> MSGIALSRLAQERKAWRKDHPFGFVAVPTKNPDGTMNLMNWECAIPGKKGTPWEGGLFKLRMLFKDDYPSSPPKCKFEPPLFHPNVYPSGTVCLSILEEDKDWRPAITIKQILLGIQELLNEPNIQDPAQ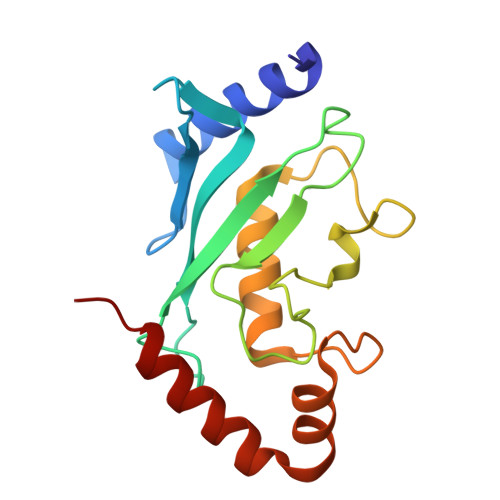AEAYTIYCQNRVEYEKRVRAQAKKFAPS> GSHMSMYNMDLDKVIRKINKKGARTVGLQFPEGLKMQAVKIAKAIESQTPATVIISGDPCFGACDVSDYKMKGSVDLIVHYGHTPLPLKYEVPTLFIEAFSNIDVKKDLEKCLEKLEDYSKI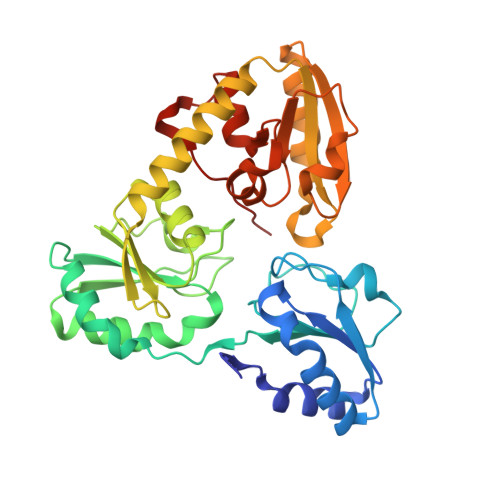ALVTTTQHLHLLNEIKDYLEDNGKEVVLGSSKNTKKGQVLGCNFSSIKNLDAEVYLFIGSGNFHPLGIYLFTKSPVLALDPYNSEIRDISAFADRILRIRFARITKAREAEKWGIIVSSKEGQYRMKLAKEIKKILEDNKMEAYIIMADNINPDILLPYMELDAFVVSACPRIAIDDSQMYKKPLLTPQELEIVLNKRQWENYQLDEILFHERYK> MAGNAYSDEVLGATN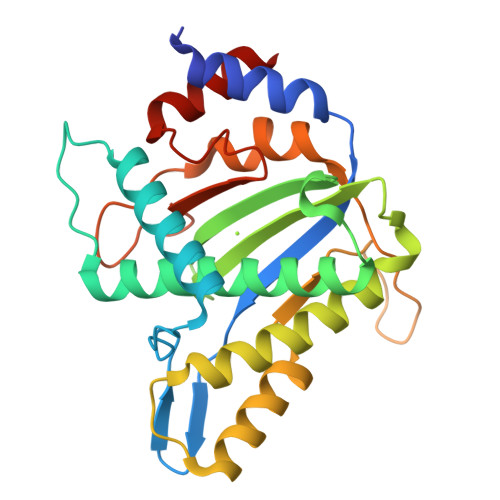WLKEKSNQEVFSFVFKNENVQLNGKDIGWNSYKKELQEDELKSLQRGAETTWDQSEDMEWETTVDEMTKKQVFIFDSLVKKCLFEVLNTKNIFPGDVNWFVQHEWGKDQGWHCHVLIGGKDFSQAQGKWWRRQLNVYWSRWLVTACNVQLTPAERIKLREIAEDNEWVTLLTYKHKQTKKDYTKCVLFGNMIAYYFLTKKKISTSPPRDGGYFLSSDSGWKTNFLKEGERHLVSKLYTDD>[3x]SNTKTASTGFAELLKDRREQVKMDHAALASLLGETPETVAAWENGEGGEL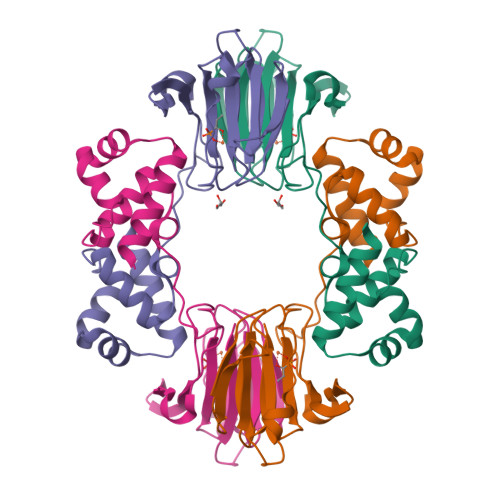TLTQLGRIAHVLGTSIGALTPPAGNDLDDGVIIQMPDERPILKGVRDNVDYYVYNCLVRTKRAPSLVPLVVDVLTDNPDDAKFNSGHAGNEFLFVLEGEIHMKWGDKENPKEALLPTGASMFVEEHVPHAFTAAKGTGSAKLIAVNF> KAFPVLGIDYTHVRTPFEISLWILLACLMKIGFHVIPTISSIVPESCLLIVVGLLVGGLIKGVGETPPFLQSDVFFLFLLPPIILDAGYFLPLRQFTENLGTILIFAVVGTLWNAFFLGGLMYAVCLVGGEQINNIGLLDNLLFGSIISAVDPVAVLAVF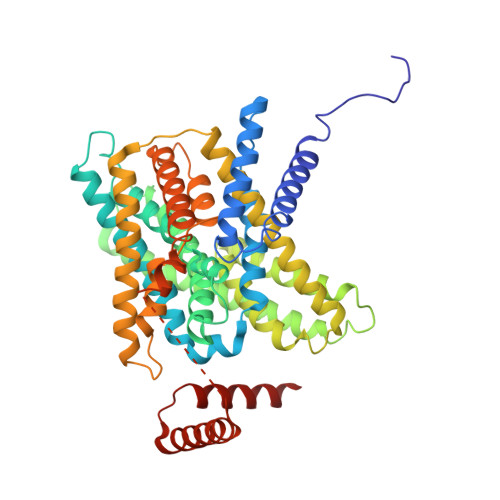EEIHINELLHILVFGESLLNDAVTVVLYHLFEEFANYEHVGIVDIFLGFLSFFVVALGGVLVGVVYGVIAAFTSRFTSHIRVIEPLFVFLYSYMAYLSAELFHLSGIMALIASGVVMRPYVEANISHKSHTTIKYFLKMWSSVSETLIFIFLGVSTVAGSHHWNWTFVISTLLFCLIARVLGVLGLTWFINKFRIVKLTPKDQFIIAYGGLRGAIAFSLGYLLDKKHFPMCDLFLTAIITVIFFTVFVQGMTIRPLVDLLAVKKKQETKRSINEEIHTQFLDHLLTGIEDICGHYGHHHWKDKLNRFNKKYV> MANVWGVRLADSLSSPTIETRTRQYTLHDLCSDLDANPGREPWKPLRNQRTNNIVAVQLFRPLQGLVLDTQLYGFPGAFDDWERFMREKLRVLKYEVLRIYPISNYSNEHVNVFVANALVGAFLSNQAFYDLLPLLIINDTMIGDLLGTGASLSQFFQSHGDVLEVAAGRKYLQMENYSNDDDDPPLFAKDLSDYAKAFYSDTYEVLDRFFWTHDSSAGVLVHYDKPTNGHHYLLGTLTQMVSAPPYIINATDAMLLESCLEQFSANVRARPAQPVTRLDQCYHLRWGAQYVGEDSLTYRLGVLSLLATNGYQLARPIPRQLTNRWLSSFVSQIMSDGVNETPLWPQERYVQIAYDSPSVVDGATQYGYVRKNQLRLGMRISALQSLSDTPSPVQWLPQYTIDQAAMDEGDLMVSRLTQLPLRPDYGNIWVGDALSYYVDYNRSHRVVLSSELPQLPDTYFDGDEQYGRSLFSLARKIGDRSLVKDTAVLKHAYQAIDPNTGKEYLRSRQSVAYFGASAGHSGADQPLVIEPWIQGKISGVPPPSSVRQFGYDVARGAIVDLARPFPSGDYQFVYSDVDQVVDGHDDLSISSGLVESLLSSCMHATAPGGSFVVKINFPTRPVWHYIEQKILPNITSYMLIKPFVTNNVELFFVAFGVHQHSSLTWTSGVYFFLVDHFYRYETLSTISRQLPSFGYVDDGSSVTGIETISIENPGFSNMTQAARIGISGLCANVGNARKSIAIYESHGARVLTITSRRSPASARRKSRLRYLPLIDPRSLEVQARTILPADPVLFENVSGASPHVCLTMMYNFEVSSAVYDGDVVLDLGTGPEAKILELIPATSPVTCVDIRPTAQPSGCWNVRTTFLELDYLSDGWITGVRGDIVTCMLSLGAAAAGKSMTFDAAFQQLIKVLSKSTANVVLVQVNCPTDVVRSIKGYLEIDSTNKRYRFPKFGRDEPYSDMDALEKICRTAWPNCSITWVPLSYDLRWTRLALLESTTLSSASIRIAELMYKYMPIMRIDIHGLPMEKRGNFIVGQNCSLVIPGFNAQDVFNCYFNSALAFSTEDVNAAMIPQVSAQFDATKGEWTLDMVFSDAGIYTMQALVGSNANPVSLGSFVVDSPDVDIT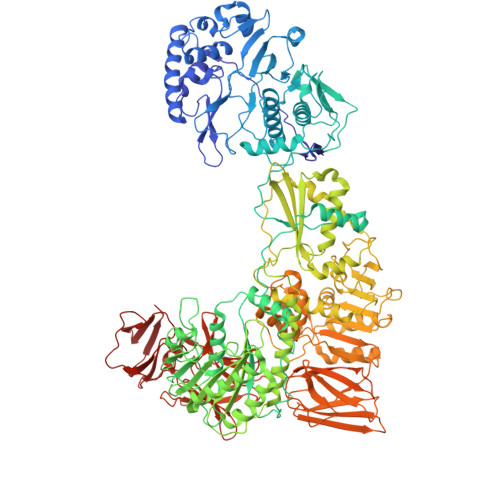DAWPAQLDFTIAGTDVDITVNPYYRLMTFVRIDGQWQIANPDKFQFFSSASGTLVMNVKLDIADKYLLYYIRDVQSRDVGFYIQHPLQLLNTITLPTNEDLFLSAPDMREWAVKESGNTICILNSQGFVLPQDWDVLTDTISWSPSIPTYIVPPGDYTLTPL>[2x]MERPQPDSMPQDLSEALKEATKEVHTQAENAEFMRNFQKGQVTRDGFKLVMASLYHIYVALEEEIERNKESPVFAPVYFPEELHRK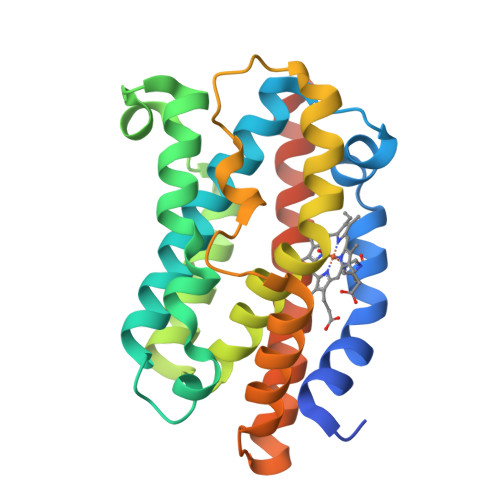AALEQDLAFWYGPRWQEVIPYTPAMQRYVKRLHEVGRTEPELLVAHAYTRYLGDLSGGQVLKKIAQKALDLPSSGEGLAFFTFPNIASATKFKQLYESRMNSLEMTPAVRQRVIEEAKTAFLLNIQLFEELQELLTHDTKDQSPSRA The initial step involved in oxidative hydroxylation of monoaromatic and polyaromatic compounds by the microorganism Sphingobium yanoikuyae strain B1 (B1), previously known as Sphingomonas yanoikuyae strain B1 and Beijerinckia sp. strain B1, is performed by a set of multiple terminal Rieske non-heme iron oxygenases. These enzymes share a single electron donor system consisting of a reductase and a ferredoxin (BPDO-FB1). One of the terminal Rieske oxygenases, biphenyl 2,3-dioxygenase (BPDO-OB1), is responsible for B1's ability to dihydroxylate large aromatic compounds, such as chrysene and benzo[a]pyrene. Rieske oxygenase systems have multiple components whose function is to transfer electrons from NAD(P)H to active molecular oxygen and ultimately oxidize aromatic hydrocarbon substrates.

The asymmetric unit contains two copies of the BPDO-FB1 molecule. The final model contains residues 3 – 104 in chains A and B. The structure has been refined to a resolution of 1.9 Å with a final Rfactor of 19.3% and an Rfree of 24.0%. The structure of the biphenyl dioxygenase system's ferredoxin component, BPDO-FB1, is the fourth Rieske oxygenase ferredoxin structure to be determined and shares significant sequence and structural homology with these proteins. BPDO-FB1 has structural features similar to other ferredoxins including three stacked beta sheets and a solvent exposed Rieske cluster. In addition to the conserved CXH-CXXH motif present in all Rieske ferredoxins, there are two additional conserved residues, Phe-71 and Pro-82, in the dioxygenase ferredoxins. The conserved proline is located at a hairpin turn at the apex of the ferredoxin and has previously been classified as part of a polyproline loop in Rieske ferredoxins. Unlike the biphenyl ferredoxin from LB400, which has three consecutive prolines, this ferredoxin has only a single proline in the loop. BPDO-FB1 is the ideal protein for exploring these effects; unlike the other Rieske oxygenase ferredoxins, this protein contains a residue which hydrogen bonds to the cluster through the side-chain, as opposed to through the main-chain as present in other ferredoxins. Thus substitution of Cys-83 with alanine, valine, or serine, can probe the effect of local charge and hydrogen bonding on the reduction potential. While the Rieske ferredoxin structure is very similar to other Rieske ferredoxins, the differences in amino acid composition near the cluster in BPDO-FB1 provide a unique opportunity among the Rieske oxygenase ferredoxins to examine the effect of cluster environment and hydrogen bonding on reduction potential.

>MSNKLRLCQVASVKDGEPVAVYQEKMPALAVYNVDGEVFVTDNLCTHGNAMLTDGYQDGTIIECPFHGGSFDIATGAAKAFPCQIPIKTYPVTIEDGWVCIDQPKESA[2x]> ENLKPPENIDVYIIDDNYTLKWSSHGESMGSVTFSAEYRTKDEAKWLKVPECQHTTTTKCEFSLLDTNVYIKTQFRVRAEEGNSTSSWNEVDPFIPF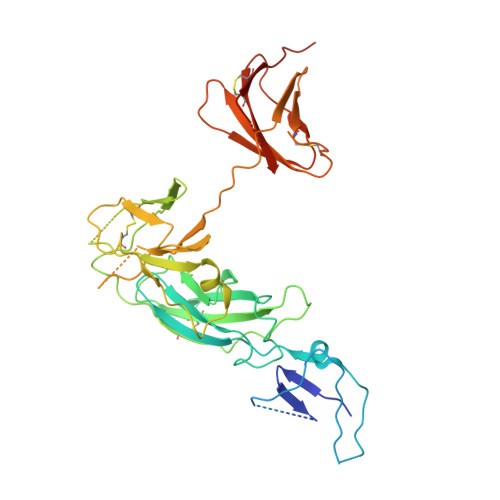YTAHMSPPEVRLEAEDKAILVHISPPGQDGNMWALEKPSFSYTIRIWQKSSSDKKTINSTYYVEKIPELLPETTYCLEVKAIHPSLKKHSNYSTVQCISTTVANKMPVPGNLQVDAQGKSYVLKWDYIASADVLFRAQWLPGYSKSSSGSRSDKWKPIPTCANVQTTHCVFSQDTVYTGTFFLHVQASEGNHTSFWSEEKFIDSQKHILPPPPVITVTAMSDTLLVYVNCQDSTCDGLNYEIIFWENTSNTKISMEKDGPEFTLKNLQPLTVYCVQARVLFRALLNKTSNFSEKLCEKTRPGSFST>[6x]INKINLNKPIIENKNNVDVSIKRYNNFVDIARLSIQKHFEHLSN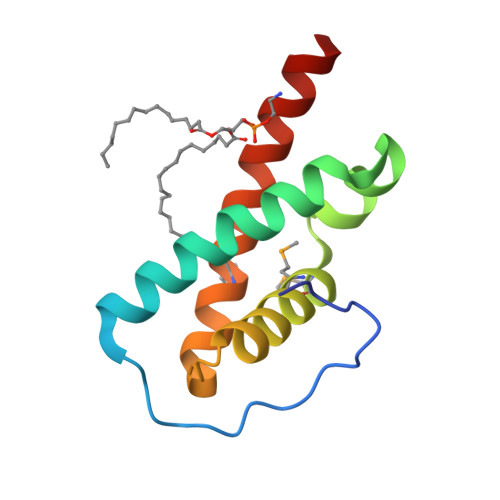DQKDSHVNNMEYMQKFVQGLQENRNISLSKYQENKAVMDLKYHLQKVYANYLSQEEN>[2x]MGSSHHHHHHSSGRENLYFQGHMPVMQSRIIHLSVEKPWAEVYDFAANPGNMPRWAAGLAGGLE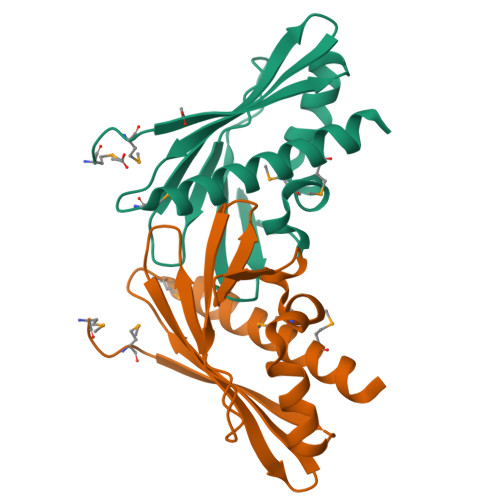ADGEDWIAKGGPLGEVRVNFAPHNEFGVIDHVVTLPDGLKVYNALRVTPNGSGTEVSFTLLRLEGMTDEDFEQDASAITADLEMLKSLLEAD>[2x]GPMSEVNVTKVIVNNPICDILDPFVFTIEFEALNKLEADLEWKIFYISAVNNEGESNQDIELDNIFLGPIERGVMMFDYAVNPPDYKN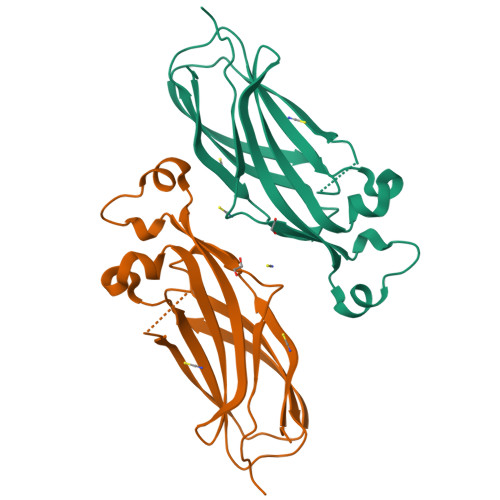MDIDSVLGLQAILISANYKEKEFIRIAYYMNSFYKDMELRENPPVVPQYDKICRHIFVENPRIVKFSIGWDSE7-(diethylamino)-3-(thiophen-2-ylcarbonyl)-2H-chromen-2-one 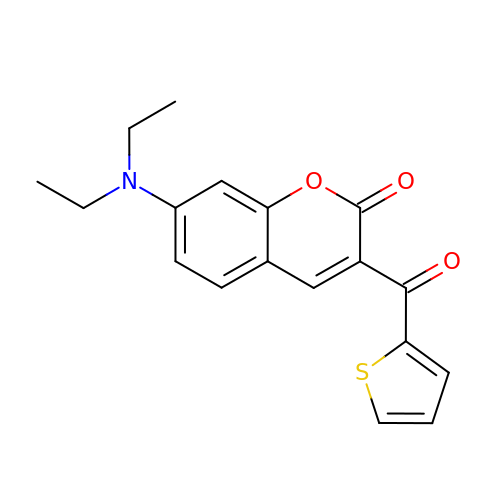| C18 H17 N O3 S | HSYRYXPRQYPBBQ-UHFFFAOYSA-N> HMSEPRFVHLHVHSDYSMIDGLAKTAPLVKKAAALGMPALAITDHTNLCGLVKFYGAGHGAGIKPIVGADFNVQCDLLGDELTHLTVLAANNTGYQNLTLLISKAYQRGYGAAGPIIDRDWLIELNEGLILLSGGRMGDVGRSLLRGNSALVDECVAFYEEHFPDRYFLELIRTGRPDEESYLHAAVELAEARGLPVVATNDVHFIDSSDFDAHEIRVAIHDGFTLDDPKRPRNYSPQQYMRSEEEMCELFADIPEALANTVEIAKRCNVTVRLGEYFLPQFPTGDMSTEDYLVKRAKEGLEERLAFLFPDEEERLKRRPEYDERLETELQVINQMGFPGYFLIVMEFIQWSKDNGVPVGPGRGSGAGSLVAYALKITDLDPLEFDLLFERFLNPERVSMPDFDVDFCMEKRDQVIEHVADMYGRDAVSQIITFGTMAAKAVIRDVGRVLGHPYGFVDRISKLIPPDPGMTLAKAFEAEPQLPEIYEADEEVKALIDMARKLEGVTRNAGKHAGGVVIAPTKITDFAPLYCDEEGKHPVTQFDKSDVEYAGLVKFDFLGLRTLTIINWALEMINKRRAKNGEPPLDIAAIPLDDKKSFDMLQRSETTAVFQLESRGMKDLIKRLQPDCFEDMIALVALFRPGPLQSGMVDNFIDRKHGREEISYPDVQWQHESLKPVLEPTYGIILYQEQVMQIAQVLSGYTLGGADMLRRAMGKKKPEEMAKQRSVFAEGAEKNGINAELAMKIFDLVEKFAGYGFNKSHSAAYALVSYQTLWLKAHYPAEFMAAVMTADMDNTEKVVGLVDECWRMGLKILPPDINSGLYHFHVNDDGEIVYGIGAIKGVGEGPIEAIIEARNKGGYFRELFDLCARTDTKKLNRRVLEKLIMSGAFDRLGPHR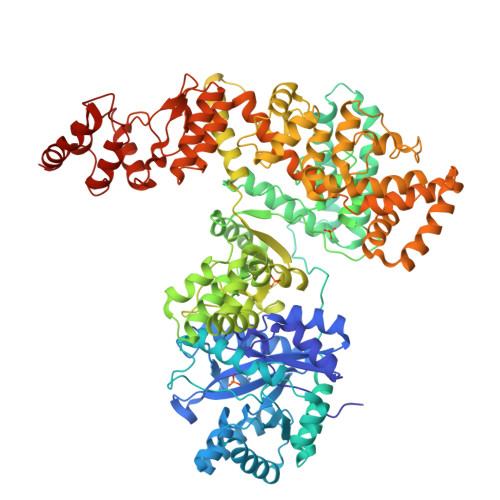AALMNSLGDALKAADQHAKAEA>MNDFHRDTWAEVDLDAIYDNVENLRRLLPDDTHIMAVVKANAYGHGDVQVARTALEAGASRLAVAFLDEALALREKGIEAPILVLGASRPADAALAAQQRIALTVFRSDWLEEASALYSGPFPIHFHLKMDTGMGRLGVKDEEETKRIVALIERHPHFVLEGLYTHFATADEVNTDYFSYQYTRFLHMLEWLPSRPPLVHCANSAASLRFPDRTFNMVRFGIAMYGLAPSPGIKPLLPYPLKEAFSLHSRLVHVKKLQPGEKVSYGATYTAQTEEWIGTIPIGYADGWLRRLQHFHVLVDGQKAPIVGRICMDQCMIRLP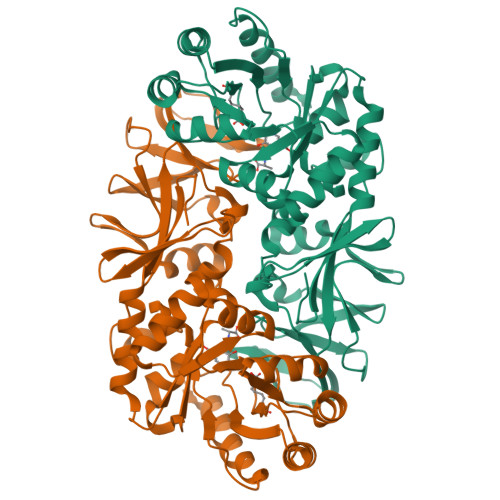GPLPVGTKVTLIGRQGDEVISIDDVARHLETINYEVPCTISYRVPRIFFRHKRIMEVRNAIGRGESSA[2x]>[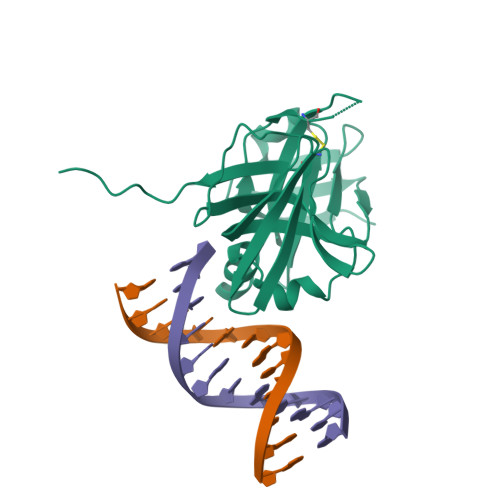2x]MDPLVVTVLKAINPFECETQEGRQEIFHATVATETDFFFVKVLNAQFKDKFIPKRTIKISNYLWHSNFMEVTSSSVVVDVESNHEVPNNVVKRARETPRISKLKIQPCGTIVNGLFKVQKITEEKDRVLYGIHDKTGTMEVLVLGNPSKTKCEEGDKIRLTFFEVSKNGVKIQLKSGPCSFFKVIKAAKPKTD> GAMGTTDDVDPEAEYAAWKLRELRRLRRERDAIEARERELAELERRRNLTEEERRAEDEAHLAKQKAEK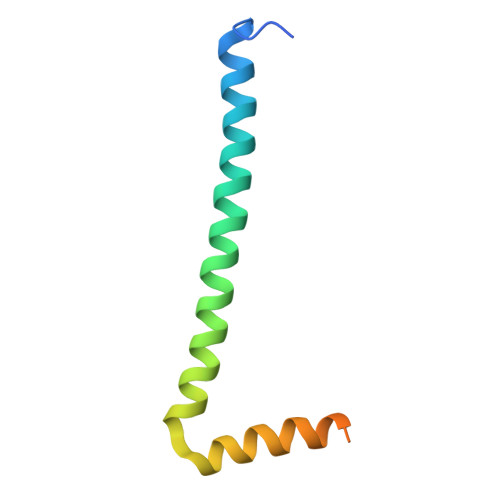ESRGKMGYLQKYFHR> MLKQVEIFTDGSCLGNPGPGGYGAILRYRGREKTFSAGYTRTTNNRMELMAAIVALEALKEHCEVILSTDSQYVRQGITQWIHNWKKRGWKTADKKPVKNVDLWQRLDAALGQHQIKWEWVKGHAGHPENERCDELARAAAMNPTLEDTGYQ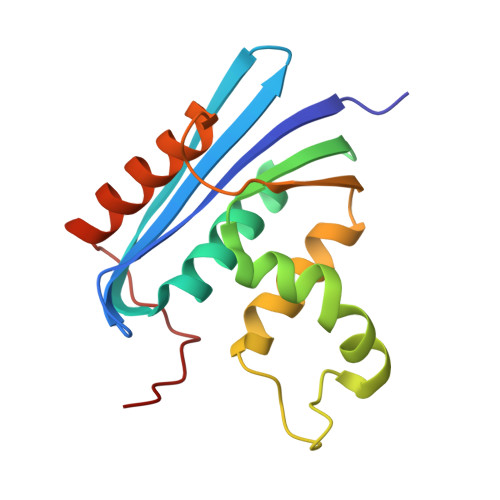VEV(5R)-5-[(1R)-1-{[6-(1-methyl-1H-pyrazol-4-yl)-2,1-benzothiazol-4-yl]oxy}ethyl]-1,3-oxazolidin-2-one 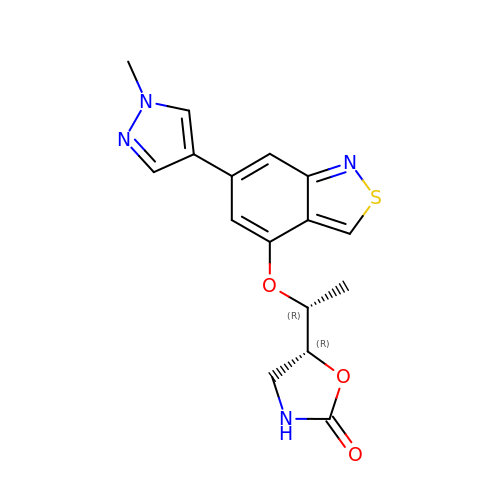| C16 H16 N4 O3 S | MKTGBKHCRFUALQ-RFAUZJTJSA-N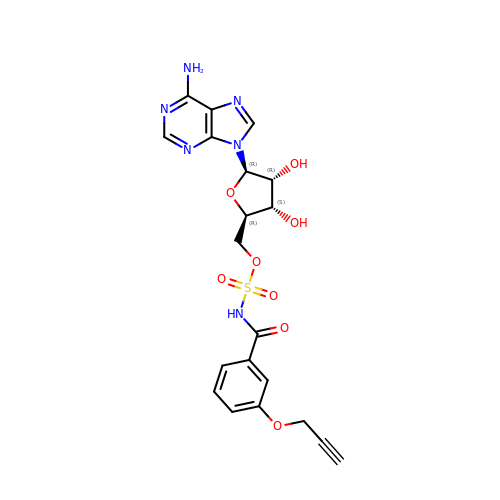[(2~{R},3~{S},4~{R},5~{R})-5-(6-aminopurin-9-yl)-3,4-bis(oxidanyl)oxolan-2-yl]methyl ~{N}-(3-prop-2-ynoxyphenyl)carbonylsulfamate | C20 H20 N6 O8 S | CEBNTACPQUEIBR-KHTYJDQRSA-N>TLYIQGQDEYYMARALKLAQRGRFTTHPNPNVGCVIVKDGEIVGEGYHQRAGEPHAEVHALRMAGEKAKGATAYVTLEPCSHHGRTPPCCDALIAAGVARVVASMQDPNPQVAGRGLYRLQQAGIDVSHGLMMSEAEQLNKGFLKRMRTGFPYIQLKLGASLDGRTAMASGESQWITSPQARRDVQLLRAQSHAILTSSATVLADDPALTVRWSELDEQTQALYPQQNLRQPIRIVIDSQNRVTPVHRIVQQPGETWFARTQEDSREWPETVRTLLIPEHKGHLDLVVLMMQLGKQQINSIWVEAGPTLAGALLQAGLVDELIVYIAPKLLGSDARGLCTLPGLEKL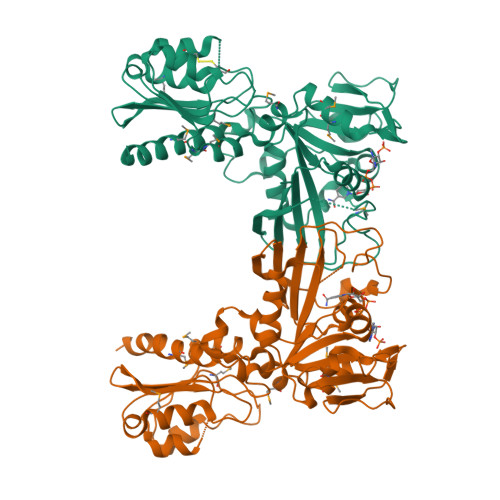ADAPQFKFKEIRHVGPDVCLHLVGASTHHHHHH[2x]3-[(E)-2-(4-hydroxyphenyl)ethenyl]-5-methoxy-phenol | C15 H14 O3 | 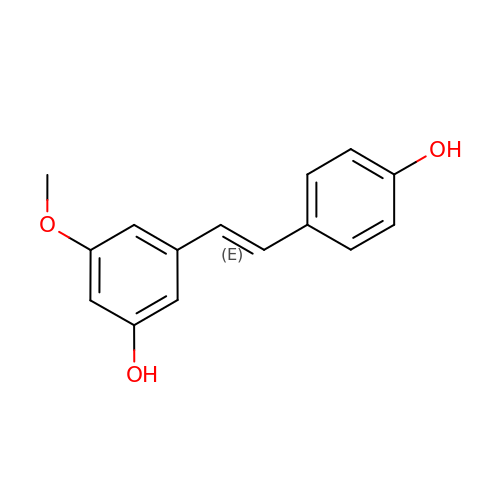KUWZXOMQXYWKBS-NSCUHMNNSA-N>[2x]MQIGKVQGRTISEFGDPAGGLKRKISTDGKNRKELPAHLSSDPKALIGQWISGIDKIYRKPDSRKSDGKAIHSPTPSKMQFDARDDLGEAFWKLVSEAGLAQDSDYDQFKRRLHPYGDKFQPADSGAKLKFEADPPEPQAFHGRWYGAMSKRGNDAKELAAALYEHLHVDEKRIDGQPKRNPKTDKFAPGLVVARALGIESSVLPRGMARLARNWGEEEIQTYFVVDVAASVKEVAKAAVSAAQAFDPPRQVSGRSLSPKVGFALAEHLERVTGSKRCSFDPAAGPSVLALHDEVKKTYKRLCARGKNAARAFPADKTELLALMRHTHENRVRNQMVRMGRVSEYRGQQAGDLAQSHYWTSAGQTEIKESEIFVRLWVGAFALAGRSMKAWIDPMGKIVNTEKNDRDLTAAVNIRQVISNKEMVAEAMARRGIYFGETPELDRLGAEGNEGFVFALLRYLRGCRNQTFHLGARAGFLKEIRKELEKTRWGKAKEAEHVVLTDKTVAAIRAIIDNDAKALGARLLADLSGAFVAHYASKEHFSTLYSEIVKAVKDAPEVSSGLPRLKLLLKRADGVRGYVHGLRDTRKHAFATKLPPPPAPRELDDPATKARYIALLRLYDGPFRAYASGITGTALAGPAARAKEAATALAQSVNVTKAYSDVMEGRTSRLRPPNDGETLREYLSALTGETATEFRVQIGYESDSENARKQAEFIENYRRDMLAFMFEDYIRAKGFDWILKIEPGATAMTRAPVLPEPIDTRGQYEHWQAALYLVM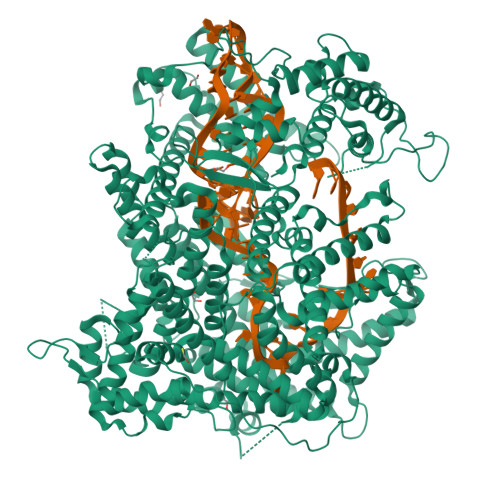HFVPASDVSNLLHQLRKWEALQGKYELVQDGDATDQADARREALDLVKRFRDVLVLFLKTGEARFEGRAAPFDLKPFRALFANPATFDRLFMATPTTARPAEDDPEGDGASEPELRVARTLRGLRQIARYNHMAVLSDLFAKHKVRDEEVARLAEIEDETQEKSQIVAAQELRTDLHDKVMKCHPKTISPEERQSYAAAIKTIEEHRFLVGRVYLGDHLRLHRLMMDVIGRLIDYAGAYERDTGTFLINASKQLGAGADWAVTIAGAANTDARTQTRKDLAHFNVLDRADGTPDLTALVNRAREMMAYDRKRKNAVPRSILDMLARLGLTLKWQMKDHLLQDATITQAAIKHLDKVRLTVGGPAAVTEARFSQDYLQMVAAVFNGSVQNPKPRRRDDGDAWHKPPKPATAQSQPDQKPPNKAPSAGSRLPPPQVGEVYEGVVVKVIDTGSLGFLAVEGVAGNIGLHISRLRRIREDAIIVGRRYRFRVEIYVPPKSNTSKLNAADLVRIDENLYFQKLAAALEHHHHHH>MANEIAALKQEIAALKKENAALKQGKLHFTYGETGKRLSELHSYHSSLTCFSEGTKVPAWGCCPASWKSFGSSCYFISSEEKVWSKSEQNCVEMGAHLVVFNTEAEQNFIVQQLNESFSYFLGLSDPQGNNNWQWIDKTPYEKNVRFWHLGEPNHSAEQCASIVFWKPTGWGWNDVICETRRNSICEMNKIYL[2x]

The sugar-binding receptors dectin-2 and blood dendritic cell antigen 2 (BDCA-2) bind oligosaccharide ligands through extracellular carbohydrate-recognition domains (CRDs) and initiate intracellular signaling through Fc receptor γ adapters (FcRγ). Dectin-2 stimulates macrophages in response to pathogen binding while BDCA-2 modulates cytokine production in plasmacytoid dendritic cells. Each of these receptors consists of an N-terminal short cytoplasmic sequence and transmembrane domain linked to a C-terminal C-type carbohydrate-recognition domain (CRD) by a short neck region. The oligomeric states of these receptors and the orientations of their CRDs have been investigated by analysis of a naturally occurring disulfide-bonded variant of BDCA-2 and by replacement of transmembrane domains with N-terminal dimerization domains to create extracellular domain dimers of both dectin-2 and BDCA-2. Analysis of these constructs, as well as previously described crystal structures of the CRDs from these proteins and a novel structure of an extended version of the extracellular domain of dectin-2, showed that there is only limited interaction of the CRDs in the dimers, but interactions can be stabilized by the presence of the neck region.

In an attempt to stabilize the conformation of the neck domain, the dectin-2 extracellular fragment beginning with residue His44 was fused to the same 3-heptad dimerization domain used with BDCA-2. This fusion product elutes in gel-filtration at the molecular weight of 44 kDa expected for a dimer. Analysis of new crystals formed by the dectin-2 dimer fused to the dimerization domain provided further insight into the interface structure. The geometry of the CRDs in crystals, which contain two dectin-2 polypeptides in the asymmetric unit, is almost identical to that observed for the isolated CRD. Two additional amino acids, SerSer at the N-terminus of each subunit, are visible in the new crystal structure. The extended interface in the new crystal expands the 4-stranded antiparallel β sheet across the dimer interface observed for the BDCA-2 and dectin-2 CRDs, contributing to a more extensive surface area of 453 Å2. The extended N-terminus introduces two more hydrogen bonds in the β-strands connecting the monomers, between Ser62 and Ser68. Additional reciprocal packing interactions can be found between Trp76 of one monomer to Leu209 and Leu64 of the other and between the Leu209 residues. Since the dimerization domain is likely to form a coiled-coil, the fact it is absent from the crystal indicates that its position is not ordered in the crystal, which in turn suggests that the neck region of dectin-2 may be flexible. The two additional serine residues visible in the new dectin-2 dimer crystals described here project to the side, indicating that the neck could bend around the CRD-CRD interface to link to the transmembrane domain.>MVKDEVIKQISTPLTSPAFPRGPYKFHNREYFNIVYRTDMDALRKVVPEPLEIDEPLVRFEIMAMHDTSGLGCYTESGQAIPVSFNGVKGDYLHMMYLDNEPAIAVGRELSAYPKKLGYPKLFVDSDTLVGTLDYGKLRVATATMGYKHKALDANEAKDQICRPNYMLKIIPNYDGSPRICELINAKITDVTVHEAWTGPTRLQLFDHAMAPL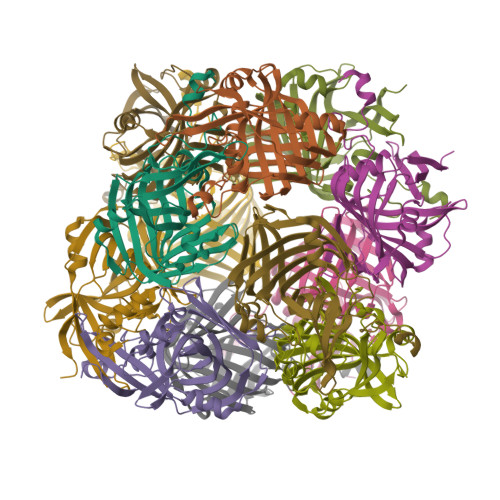NDLPVKEIVSSSHILADIILPRAEVIYDYLK[4x]> GAGATGAGAGYYI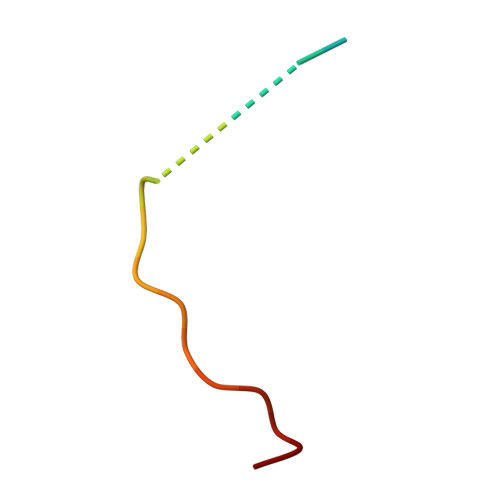TPRTGAGA>[4x]QVVSQGWKYFKGNFYYFSLIPKTWYSAEQFCVSRNSHLTSVTSESEQEFLYKTAGGLIYWIGLTKAGMEGDWSWVDDTPFNKVQSV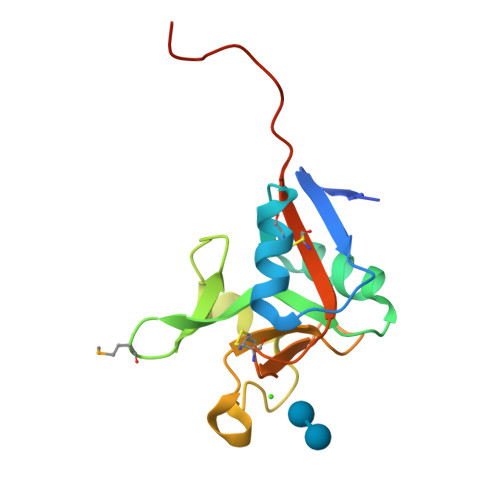RFWIPGEPNNAGNNEHCGNIKAPSLQAWNDAPCDKTFLFICKRPYVPSEPSAWSHPQFEK> ATRRYYLGAVELSWDYMQSDLGELPVDARFPPRVPKSFPFNTSVVYKKTLFVEFTDHLFNIAKPRPPWMGLLGPTIQAEVYDTVVITLKNMASHPVSLHAVGVSYWKASEGAEYDDQTSQREKEDDKVFPGGSHTYVWQVLKENGPMASDPLCLTYSYLSHVDLVKDLNSGLIGALLVCREGSLAKEKTQTLHKFILLFAVFDEGKSWHSETKNSLMQDRDAASARAWPKMHTVNGYVNRSLPGLIGCHRKSVYWHVIGMGTTPE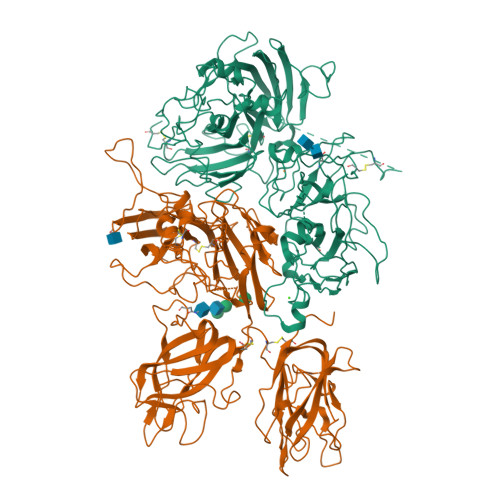VHSIFLEGHTFLVRNHRQASLEISPITFLTAQTLLMDLGQFLLFCHISSHQHDGMEAYVKVDSCPEEPQLRMKNNEEAEDYDDDLTDSEMDVVRFDDDNSPSFIQIRSVAKKHPKTWVHYIAAEEEDWDYAPLVLAPDDRSYKSQYLNNGPQRIGRKYKKVRFMAYTDETFKTREAIQHESGILGPLLYGEVGDTLLIIFKNQASRPYNIYPHGITDVRPLYSRRLPKGVKHLKDFPILPGEIFKYKWTVTVEDGPTKSDPRCLTRYYSSFVNMERDLASGLIGPLLICYKESVDQRGNQIMSDKRNVILFSVFDENRSWYLTENIQRFLPNPAGVQLEDPEFQASNIMHSINGYVFDSLQLSVCLHEVAYWYILSIGAQTDFLSVFFSGYTFKHKMVYEDTLTLFPFSGETVFMSMENPGLWILGCHNSDFRNRGMTALLKVSSCDKNTGDYYEDSYEDISAYLLSKNNAIEPRSFSQNPPVLKRHQR;> EITRTTLQSDQEEIDYDDTISVEMKKEDFDIYDEDENQSPRSFQKKTRHYFIAAVERLWDYGMSSSPHVLRNRAQSGSVPQFKKVVFQEFTDGSFTQPLYRGELNEHLGLLGPYIRAEVEDNIMVTFRNQASRPYSFYSSLISYEEDQRQGAEPRKNFVKPNETKTYFWKVQHHMAPTKDEFDCKAWAYFSDVDLEKDVHSGLIGPLLVCHTNTLNPAHGRQVTVQEFALFLTIFDETKSWYFTENMERNCRAPCNIQMEDPTFKENYRFHAINGYIMDTLPGLVMAQDQRIRWYLLSMGSNENIHSIHFSGHVFTVRKKEEYKMALYNLYPGVFETVEMLPSKAGIWRVECLIGEHLHAGMSTLFLVYSNKCQTPLGMASGHIRDFQITASGQYGQWAPKLARLHYSGSINAWSTKEPFSWIKVDLLAPMIIHGIKTQGARQKFSSLYISQFIIMYSLDGKKWQTYRGNSTGTLMVFFGNVDSSGIKHNIFNPPIIARYIRLHPTHYSIRSTLRMELMGCDLNSCSMPLGMESKAISDAQITASSYFTNMFATWSPSKARLHLQGRSNAWRPQVNNPKEWLQVDFQKTMKVTGVTTQGVKSLLTSMYVKEFLISSSQDGHQWTLFFQNGKVKVFQGNQDSFTPVVNSLDPPLLTRYLRIHPQSWVHQIALRMEVLGCEAQDLY>NNTLWTGPKPEANCIIEYGKQNPDSKLTLILVKNGGIVNGYVTLMGASDYVNTLFKNKNVSINVELYFDATGHILPDSSSLKTDLELKYKQTADFSARGFMPSTTAYPFVLPNGTHNENYIFGQCYYKASDGALFPLE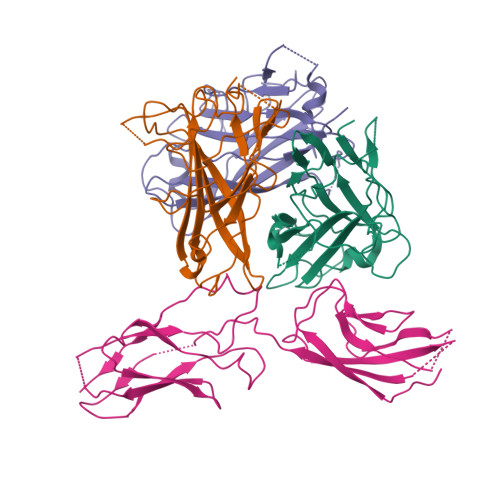VTVMLNKRLPDSRTSYVMTFLWSLNAGLAPETTQATLITSPFTFSYIRED[3x];> PVFTQDVFVGSVEELSAAHTLVMKINATDAEPNTLSKISYRIVSLEPAYPPVFYLNKDTGEIYTTSVTLDREEHSSYTLTVEARDGVKQAQVQIRILDVNDNIPVVELEGMVEENQVNVEVTRIKVFDADEIGSDNWLANFTFASGNEGGYFHIETDAQTNEGIVTLIKEVYMKNLDFSVIVANKAAFHKSIRSKYKPTPIPIKVKVK> MSGEE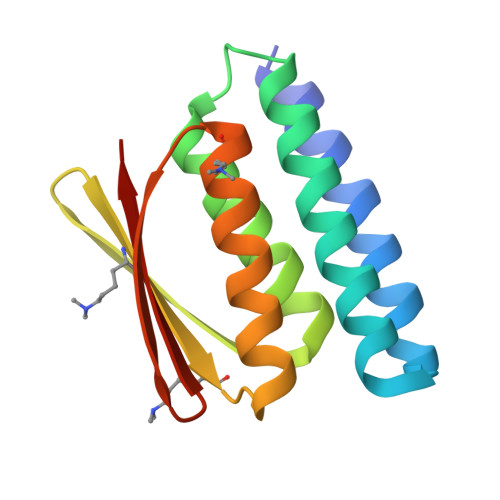AVRRRFEELLREALAFRERTGGRRETLEHAVRLARELAEFAASHPEFNRQEAVLLAIELMVRAMGVTMETHRSGNEVKVVIKGLNIDEQVALYRAVRETSKIMGVETEIEVEGDTQTIVVREGSG ethyl 4-(5,6,7,8-tetrahydroacridin-3-ylcarbonyl)piperazine-1-carboxylate | C21 H25 N3 O3 | 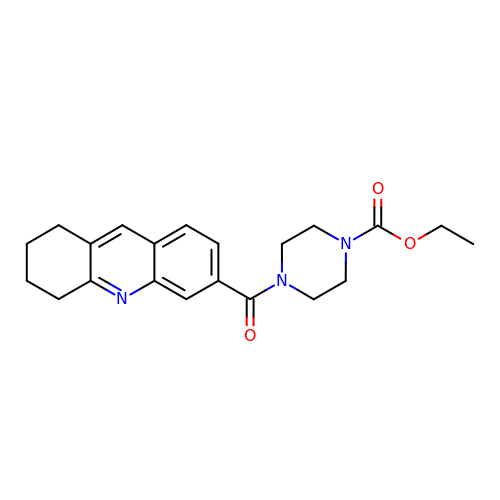YMYFCDFYTNCCDJ-UHFFFAOYSA-N HYPOXANTHINE | C5 H4 N4 O | 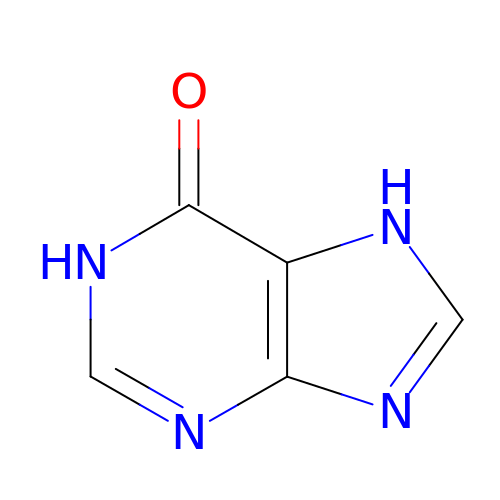FDGQSTZJBFJUBT-UHFFFAOYSA-N>[4x]MTSIQQRDAQSVLAAIDNLLPEIRDRAQATEDLRRLPDETVKALDDVGFFTLLQPQQWGGLQCDPALFFEATRRLASV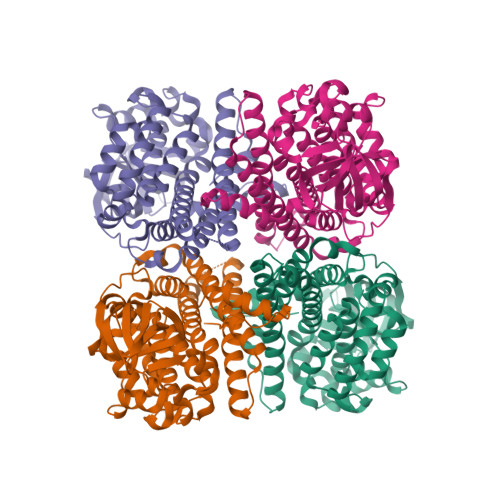CGSTGWVSSIVGVHNWHLALFDQRAQEEVWGEDPSTRISSSYAPMGAGVVVDGGYLVNGSWNWSSGCDHASWTFVGGPVIKDGRPVDFGSFLIPRSEYEIKDVWYVVGLRGTGSNTLVVKDVFVPRHRFLSYKAMNDHTAGGLATNSAPVYKMPWGTMHPTTISAPIVGMAYGAYAAHVEHQGKRVRAAFAGEKAKDDPFAKVRIAEAASDIDAAWRQLIGNVSDEYALLAAGKEIPFELRARARRDQVRATGRSIASIDRLFEASGATALSNEAPIQRFWRDAHAGRVHAANDPERAYVIFGNHEFGLPPGDTMV>[2x]MTLQYTALGDSLTVGVGAGLFEPGFVQRYKRKMEEDLNEEVSLIVFAKSGLETSEILAMLNEPFIMEQVKKADVITITGCGNDLLQSLEIYE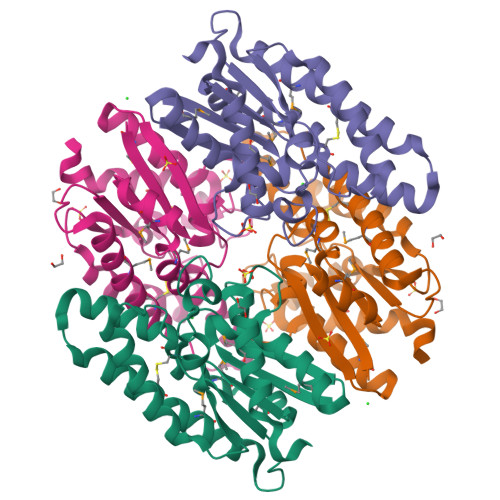KEKDEHVFLEASSHCQKNYSGMLEKIREIKGEKDTRYLVRLLNLYNPFPSIELADKWISGFNRHLKQLESAPQIKVIDTYAVFKGREKEYLSIDRVHPSSRGYEAMSEKLRAAGYGRLEGHHHHHH> SRKTYTLTDYLKNTYRLKLYSLRWISDHEYLYKQENNILVFNAEYGNSSVFLENSTFDEFGHSINDYSISPDGQFILLEYNYVKQWRHSYTASYDIYDLNKRQLITEERIPNNTQWVTWSPVGHKLAYVWNNDIYVKIEPNLPSYRITWTGKEDIIYNGITDWVYEEEVFSAYSALWWSPNGTFLAYAQFNDTEVPLIEYSFYSDESLQYPKTVRVPYPKAGAVNPTVKFFVVNTDSLSSVTNATSIQITAPASMLIGDHYLCDVTWATQERISLQWLRRIQNYSVMDICDYDESSGRWNCLVARQHIEMSTTGWVGRFRPSEPHFTLDGNSFYKIISNEEGYRHICYFQIDKKDCTFITKGTWEVIGIEALTSDYLYYISNEYKGMPGGRNLYKIQLSDYTKVTCLSCELNPERCQYYSVSFSKEAKYYQLRCSGPGLPLYTLHSSVNDKGLRVLEDNSALDKMLQNVQMPSKKLDFIILNETKFWYQMILPPHFDKSKKYPLLLDVYAGPCSQKADTVFRLNWATYLASTENIIVASFDGRGSGYQGDKIMHAINRRLGTFEVEDQIEAARQFSKMGFVDNKRIAIWGWSYGGYVTSMVLGSGSGVFKCGIAVAPVSRWEYYDSVYTERYMGLPTPEDNLDHYRNSTVMSRAENFKQVEYLLIHGTADDNVHFQQSAQISKALVDVGVDFQAMWYTDEDHGIASSTAHQHIYTHMSHFIKQCFSLPHHHHHH;> EAAATGTFIEQPKSKECDFTPMLVGVPPQVYNFKRLVFTNCNYNLTKLLSLFMVNEFSCNGISPDAIARGCYSSLTVDYFAYPLSMRSYIQPGSAGDISLYNYKQSFANPTCRVLATAPANLTLTKPSAYGYFQKCSRVSGEHNSVETPLYINPGEYSICRSFSPYGFSEDGEVFRRQLTQYEGGGILVGVGAKLAMTDKLEMGFIISVQYGTDTNSVCPMLDLGNSSTITHYLGKCVDYHHHHHH

A novel pangolin-origin MERS-like coronavirus (CoV), MjHKU4r-CoV-1, was recently identified. MjHKU4r-CoV-1 uses the dipeptidyl peptidase 4 (DPP4 or CD26) receptor for virus entry and has a broad host tropism. The receptor recognition of coronaviruses is mediated by the spike (S) protein on the viral envelope, which modulates host and tissue tropism, pathogenicity, and zoonotic transmission. Recently reported MjHKU4r-CoV-1 also uses its RBD to interact with CD26 for virus entry.

Structural analysis revealed that residues Y463, K509, H517, N518, E521, S543, D545, E547, and R550 of the MjHKU4r-CoV-1 RBD form an extensive H-bond network with residues K267, T288, A289, A291, L294, R317, R336, and Q344 of hCD26. Notably, the N-glycans of N229 on hCD26 were observed to form more extensive hydrophilic interactions with the MjHKU4r-CoV-1 RBD than that observed in the HKU4-CoV RBD/hCD26 and MERS-CoV RBD/hCD26 complex structures. Furthermore, there is a hydrophobic pocket formed by residues V513, V548, V565, I561, and V563 of the MjHKU4r-CoV-1 RBD, and a helix on hCD26 formed by A289, P290, A291, S292, M293, L294, I295, and G296 inserts into this groove. Residues A291, L294, and I295 of hCD26 form extensive hydrophobic interactions with the hydrophobic pocket. Notably, the interface formed by residues S502, F537, S538, Y540, G541, F542 and F549 of the MjHKU4r-CoV-1 RBD interacts with the N-glycans of N229 in hCD26, which is not observed in the HKU4-CoV RBD/hCD26 and MERS-CoV RBD/hCD26 complexes due to the shorter N-glycans resulting from different protein expression systems. In this work, a mammalian expression system was used for hCD26 expression. However, the structural alignment shows that the MjHKU4r-CoV-1 RBD is closer to hCD26 and its N229 N-glycans than the HKU4-CoV and MERS-CoV RBDs (Fig. EV2), suggesting that the MjHKU4r-CoV-1 RBD forms stronger interactions to bind more tightly to hCD26 than the other two RBDs. The binding affinity between the MjHKU4r-CoV-1 RBD and hCD26 harboring T288A or Q344A mutations was ~0.35 μM or 0.28 µM, respectively, similar to that between the wild-type MjHKU4r-CoV-1 RBD and hCD26. The above results indicate that the side chains of residues K267, R317 and R336 are crucial for hCD26 binding to the MjHKU4r-CoV-1 RBD. Thus, the lack of binding affinity of cat CD26 for the MjHKU4r-CoV-1 RBD is the comprehensive impact caused by differential AAs, mainly contributed by residues A292, T295, K336, and E344 at the RBD-CD26 interface. The above results implicate that residue sites 291, 292, 294, 295, 336, and 344 of CD26 are crucial for determining their capacity to bind the MjHKU4r-CoV-1 RBD.>MSQFFIRRPVFAWVIAIFIIIFGLLSIPKLPIARFPSVAPPQVNISATYPGATAKTINDSVVTLIERELSGVKNLLYYSATTDTSGTAEITATFKPGTDVEMAQVDVQNKIKAVEARLPQVVRQQGLQVEASSSGFLMLVGINSPNNQYSEVDLSDYLVRNVVEELKRVEGVGKVQSFGAEKAMRIWVDPNKLVSYGLSISDVNNAIRENNVEIAPGRLGDLPAEKGQLITIPLSAQGQLSSLEQFKNISLKSKTNGSVIKLSDVANVEIGSQAYNFAILENGKPATAAAIQLSPGANAVKTAEGVRAKIEELKLNLPEGMEFSIPYDTAPFVKISIEKVIHTLLEAMVLVFIVMYLFLHNVRYTLIPAIVAPIALLGTFTVMLLAGFSINVLTMFGMVLAIGIIVDDAIVVVENVERIMATEGLSPKDATSKAMKEITSPIIGITLVLAAVFLPMAFASGSVGVIYKQFTLTMSVSILFSALLALILTPALCATILKPIDGHHQKKGFFAWFDRSFDKVTKKYELMLLKIIKHTVPMMVIFLVITGITFAGMKYWPTAFMPEEDQGWFMTSFQLPSDATAERTRNVVNQFENNLKDNPDVKSNTAILGWGFSGAGQNVAVAFTTLKDFKERTSSASKMTSDVNSSMANSTEGETMAVLPPAIDELGTFSGFSLRLQDRANLGMPALLAAQDELMAMAAKNKKFYMVWNEGLPQGDNISLKIDREKLSALGVKFSDVSDIISTSMGSMYINDFPNQGRMQQVIVQVEAKSR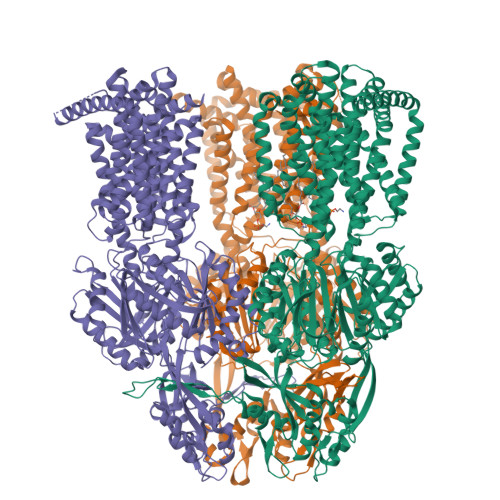MQLKDILNLKVMGSSGQLVSLSEVVTPQWNKAPQQYNRYNGRPSLSIAGIPNFDTSSGEAMREMEQLIAKLPKGIGYEWTGISLQEKQSESQMAFLLGLSMLVVFLVLAALYESWAIPLSVMLVVPLGIFGAIIAIMSRGLMNDVFFKIGLITIIGLSAKNAILIVEFAKMLKEEGMSLIEATVAAAKLRLRPILMTSLAFTCGVIPLVIATGASSETQHALGTGVFGGMISATILAIFFVPVFFIFILGAVEKLFSSKKKISS[3x]>MSSLLVKKLVESATTPMRGSEGAAGYDISSVEDVVVPAMGRIAVSTGISIRVPDGTYGRIAPRSGLAYKYGIDVLAGVIDSDYRGEVKVILYNTTERDYIIKKGDRIAQLILEQIVTPGVAVVLDLSDTARGSGGFGSTGI[4x]

dUTPase (EC 3.6.1.23) is a ubiquitous enzyme that catalyzes the hydrolysis of dUTP to diphosphate and dUMP, the substrate for thymidylate synthetase in dTTP biosynthesis. The 141-amino-acid deoxyuridine triphosphatase (dUTPase) from the algal Chlorella virus IL-3A and its Glu81Ser/Thr84Arg-mutant derivative Mu-22 were crystallized using the hanging-drop vapor-diffusion method at 298 K with polyethylene glycol as the precipitant. We previously generated Mu-22 dUTPase by mutating two IL-3A residues to the corresponding residues from PBCV-1 dUTPase. The presence of these two mutations (Glu81Ser and Thr84Arg), creating the derivative Mu-22 dUTPase, led to an increase in the optimal temperature of the enzyme to 328 K. Here, we conduct structural studies of dUTPases from Chlorella viruses in order to elucidate the molecular mechanisms behind the differences in optimal temperature.

Glycyl-seryl-tagged dUTPases yielded cubic P213 IL-3A crystals with unit-cell parameter a = 105.68 Å and hexagonal P63 Mu-22 crystals with unit-cell parameters a = 132.07, c = 53.45 Å, γ = 120°. Owing to the Thr84Arg mutation, Mu-22 dUTPase had different monomer-to-monomer interactions to those of IL-3A dUTPase.>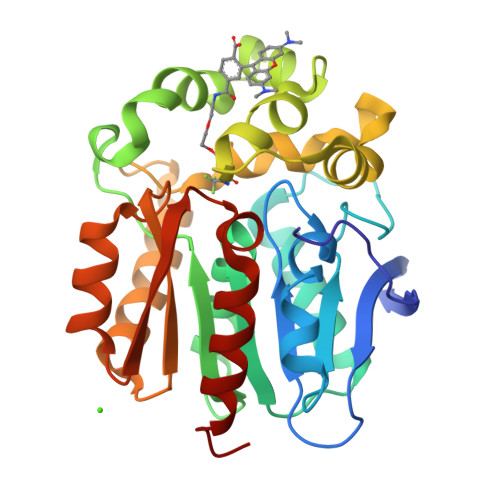[2x]GIGTGFPFDPHYVEVLGERMHYVDVGPRDGTPVLFLHGNPTSSYVWRNIIPHVAPTHRCIAPDLIGMGKSDKPDLGYFFDDHVRFMDAFIEALGLEEVVLVIHDWGSALGFHWAKRNPERVKGIAFMEFIRPIPTWDEWPEFARETFQAFRTTDVGRKLIIDQNVFIEGTLPMGVVRPLTEVEMDHYREPFLNPVDREPLWRFPNELPIAGEPANIVALVEEYMDWLHQSPVPKLLFWGTPGVLIPPAEAARLAKSLPNCKAVDIGPGLNLLQEDNPDLIGSEIARWLSTLEI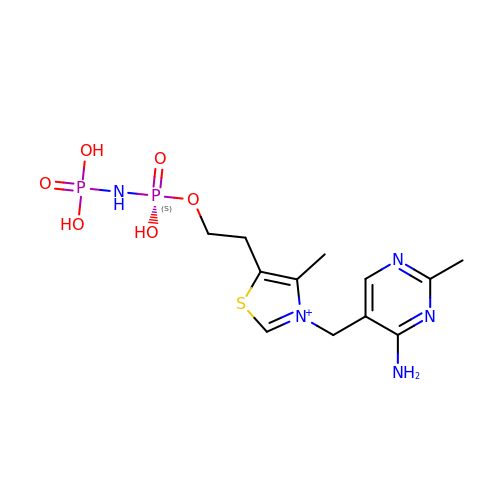3-[(4-AMINO-2-METHYLPYRIMIDIN-5-YL)METHYL]-5-(2-{[HYDROXY(PHOSPHONOAMINO)PHOSPHORYL]OXY}ETHYL)-4-METHYL-1,3-THIAZOL-3-IUM | C12 H20 N5 O6 P2 S | LWNISHVQCROCTL-UHFFFAOYSA-O> SNAFKRRRCGVCEVCQQPECGKCKACKDMVKFGGSGRSKQACQERRCPNMAMKEADDDEEVDDNIPE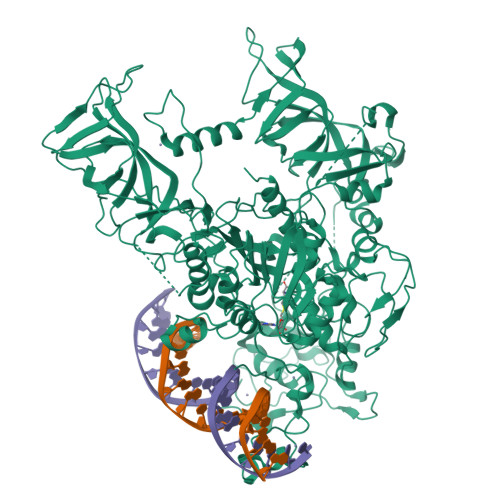MPSPKKMHQGKKKKQNKNRISWVGEAVKTDGKKSYYKKVCIDAETLEVGDCVSVIPDDSSKPLYLARVTALWEDSSNGQMFHAHWFCAGTDTVLGATSDPLELFLVDECEDMQLSYIHSKVKVIYKAPSENWAMEGGMDPESLLEGDDGKTYFYQLWYDQDYARFESPPKTQPTEDNKFKFCVSCARLAEMRQKEIPRVLEQLEDLDSRVLYYSATKNGILYRVGDGVYLPPEAFTFNIKLSSPVKRPRKEPVDEDLYPEHYRKYSDYIKGSNLDAPEPYRIGRIKEIFCPKKSNGRPNETDIKIRVNKFYRPENTHKSTPASYHADINLLYWSDEEAVVDFKAVQGRCTVEYGEDLPECVQVYSMGGPNRFYFLEAYNAKSKSFEDPPNHARSPGNKGKGKGKGKGKPKSQACEPSEPEIEIKLPKLRTLDVFSGCGGLSEGFHQAGISDTLWAIEMWDPAAQAFRLNNPGSTVFTEDCNILLKLVMAGETTNSRGQRLPQKGDVEMLCGGPPCQGFSGMNRFNSRTYSKFKNSLVVSFLSYCDYYRPRFFLLENVRNFVSFKRSMVLKLTLRCLVRMGYQCTFGVLQAGQYGVAQTRRRAIILAAAPGEKLPLFPEPLHVFAPRACQLSVVVDDKKFVSNITRLSSGPFRTITVRDTMSDLPEVRNGASALEISYNGEPQSWFQRQLRGAQYQPILRDHICKDMSALVAARMRHIPLAPGSDWRDLPNIEVRLSDGTMARKLRYTHHDRKNGRSSSGALRGVCSCVEAGKACDPAARQFNTLIPWCLPHTGNRHNHWAGLYGRLEWDGFFSTTVTNPEPMGKQGRVLHPEQHRVVSVRECARSQGFPDTYRLFGNILDKHRQVGNAVPPPLAKAIGLEIKLCMLAKA> MARSVSSLQSLCITKISENISKWQKEADESSKLVFNKLRDVLGGVSTANLNNLAKALSKNRALNDHTLQLFLKTDLKRLTFSDCSKISFDGYKTLAIFSPHLTELSLQMCGQLNHESLLYIAEKLPNLKSLNLDGPFLINEDTWEKFFVIMKGRLEEFHISNTHRFTDKSLSNLLINCGSTLVSLGLSRLDSISNYALLPQYLVNDEFHSLCIEYPFNEEDVNDEIIINLLGQIGRTLRKLVLNGCIDLTDSMIINGLTAFIPEKCPLEVLSLEESDQITTDSLSYFFSKVELNNLIECSFRRCLQLGDMAIIELLLNGARDSLRSLNLNSLKELTKEAFVALACPNLTYLDLGFVRCVDDSVIQMLGEQNPNLTVIDVFGDNLVTEKATMRPGLTLIGRQSDSI;> MGSSHHHHHHSQGSMSQDFVTLVSKDDKEYEISRSAAMISPTLKAGRIELKQFDSHILEKAVEYLNYNLKYSGVSEDDDEIP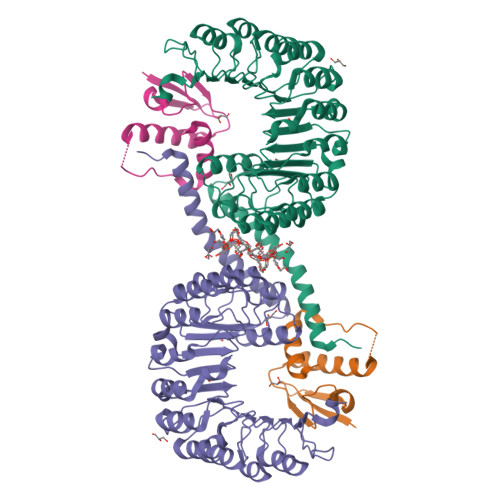EFEIPTEMSLELLLAADYLSI> MTGADGAIAKLQSYNYSHMYIRNANFDVRIDDNVTPETDAQWVLVPGLANSGEGYVSIQSVDHLGYYLRHWNYDFRLEKNDGTRIFAEDATFKMVPGLADPSYTSFQSYNYPTRYIRHYNYLLRLDEIVTALDREDATFRVIDSSSVDPDKADDSVIVTNPIVRRRADPWVYRHTDGYYYMTASVPEYDRIELRRSRTLQGLSTATPKTIWRRHSSGIMGGHIWAPEIHFIDGKWYIYFSAGTSTNYFDIRLYVLECSDSNPLTGTWVEKGQLKTNWESFTLDATTFEHNGTRYLVWAQKDPKIASNSNIYIAKMNGPLAITGNQVMISTPEYSWEKIGYAVNEGPAVLKKNGKIFITFSASATDANYCMGLLTASDTANLLDPKSWHKSPNPVFQSNPSTGQYGPGHNSFTTSPDGKVDIMVYHARNYRDITGDPLYDPNRHTRAQIVNWNADGTPDFGIPVADGTNVIYIPPQTPTPIPTNSPTPSDLIYLEHHHHHH

Here, we describe the structure and function of AtAbf43C, an uncharacterized GH family 43 subfamily 26 (GH43_26) α-L-arabinofuranosidase (EC 3.2.1.55) from A. thermocellus. We solved high-resolution crystal structures of full-length AtAbf43C and its individual carbohydrate binding module family 42 (CBM42) and GH43 domains, including a structure with L-arabinofuranose molecules bound to the CBM42. The predicted 580 amino acid protein consists of an N-terminal signal peptide (residues 1–19), a CBM42 domain (residues 29–160), a GH43 domain (residues 179–488), and a C-terminal dockerin I domain (residues 511–568). Taken together, we demonstrate through structural and functional characterization that AtAbf43C is an active arabinofuranosidase, specialized in degrading AOSs to arabinose in an exo manner.

First, the arabinose-bound structure of full-length AtAbf43C builds upon previous work by Ribeiro et al., by providing structural evidence for a nonfunctional α-binding pocket, with arabinose only bound in the β- and γ- subdomains. In addition to the two arabinose molecules bound to the CBM42 domain, the structure contains three glycerol molecules and a central magnesium ion in the GH43 domain. In the β pocket, the arabinose molecule formed hydrogen bonds with three residues, Y73, H70, and D89. Similarly, the arabinose in the γ pocket contacted Y121, H118, and D136, as well as an additional residue N120. In the previous study of this CBM42 by Ribeiro et al., residues D39, D91, and D136 were individually altered to alanine. While versions with the D91A and D136A substitutions showed significantly decreased binding affinity for arabinoxylan and arabinose relative to the wildtype protein, the D39A mutation, which corresponds to the α pocket, did not significantly affect binding. The binding pattern of arabinose observed in our structure would thus appear to support that the α pocket is nonfunctional or does not contribute to arabinose binding in the Atabf43C CBM42 domain. The binding domain of AtAbf43C also closely aligned with the CBM42 domain in SaAraf43A. However, while both structures had sugars in their β-subdomains, the SaAraf43A CBM42 had an arabinobiose bound in its α-pocket, and an unliganded γ-pocket. Furthermore, alignment of binding residues in the α-pocket differed significantly between the two proteins, with AtAbf43C possessing a proline and two glutamines at positions where SaAraf43A possesses glutamine, histidine, and aspartate residues, respectively.>GSMTEIALIGNPNSGKTSLFNLITGHNQRVGNWPGVTVERKSGLVKKNKDLEIQDLPGIYSMSPYSPEEKVARDYLLSQRADSILNVVDATNLERNLYLTTQLIETGIPVTIALNMIDVLDGQGKKINVDKLSYHLGVPVVATSALKQTGVDQVVKKAAHTTTSTVGDLAFPIYDDRLEAAISQILEVLGNSVPQRSARFYAIKLFEQDSLVEAELDLSQFQRKEIEDIIRITEEIFTEDAESIVINERYAFIERVCQMAESHTEDFALTLS[2x]

The protein is separated into three domains: An N-terminal cytoplasmic GTPase domain (G-domain), a helical domain (together with the G-domain termed ‘NFeoB’), and a C-terminal polytopic membrane-spanning domain. While the import of Fe2+ by FeoB is dependent upon GTP hydrolysis by the G-domain, the mechanism of coupling between the two events is unknown. Like other small G-proteins, the G-domain of NFeoB undergoes significant structural rearrangement in response to nucleotide binding and hydrolysis. Recently, it was shown that the rate of nucleotide hydrolysis and conformational switching by NFeoB is accelerated in the presence of potassium ions, and the protein has been classified as a member of the potassium-activated TrmE-Era-EngA-YihA-Septin-like (TEES) superfamily of G-proteins.

Crystals were obtained in space group P212121 with two molecules in the asymmetric unit, and the crystals diffracted to a resolution of 2.5 Å. The transition-state structure shows the canonical G-protein domain fold (residues 1–170) interacting with the helical domain (residues 171–270). Conversion of the GTP substrate to its transition-state causes Switch II, and the adjacent portion of the helical domain, to shift away from the nucleotide binding site. Switch I, however, remains locked its active conformation, capping the nucleotide in the same orientation observed in the mGMPPNP-bound structure. The potassium ion lies at the nucleotide binding site between the G1 P-loop and the apex of Switch I. The ligands for the potassium ion are the backbone carbonyls of Gly29 and Trp31, the sidechain amide oxygen of Asn11, one oxygen each from the β- and γ-phosphates, and one fluorine atom from the transition state analogue. The bond lengths about the potassium are long, up to 3.2 Å, which is necessitated by the strict geometric constraints imposed by the protein and the nucleotide ligands. In this way, a binding site is created which is selective for potassium rather than sodium – a smaller ion that prefers significantly shorter metal-oxygen bond lengths. In its magnesium-bound conformation, the backbone carbonyl of Thr35 hydrogen-bonds with the attacking water molecule, which is also the recipient of another hydrogen bond from the backbone amide from Gly56 from the G3 motif. Therefore, this supports the results from the current study, which suggests that water alignment in NFeoBSt is achieved only via hydrogen-bonding interactions with the backbone amides from Thr35 and Gly56, the conserved glycine residue from the G3 motif.> AECSVDIQGNDQMQFNTNAITVDKSCKQFTVNLSHPGNLPKNVMGHNWVLSTAADMQGVVTDGMASGLDKDYLKPDDSRVIAHTKLIGSGEKDS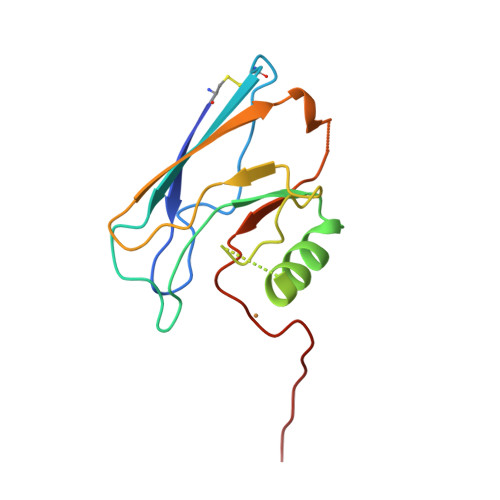VTFDVSKLKEGEQYMFFCAAAHAAAMKGTLTLK> MGSDSIDTPNYDVQKHINKLCGMLLITEDANHKFTGLIGMLYAMSRLGREDTIKILRDAGYHVKANGVDVTTHRQDINGKEMKFEVLTLASLTTEIQINIEIESRKSYKKMLKEMGEVAPEYRH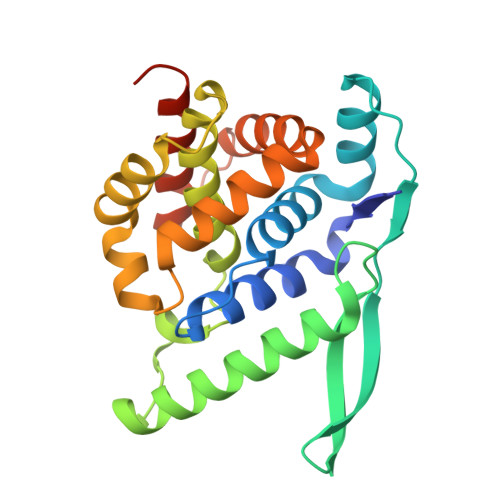DSPDCGMIILCIAALVITKLAAGDRSGLTAVIRRANNVLKNEMKRYKGLLPKDIANSFYEVFEKHPHFIDVFVHFGIAQSSTRGGSRVEGIFAGLFMNAYGLEHHHHHH>[2x]S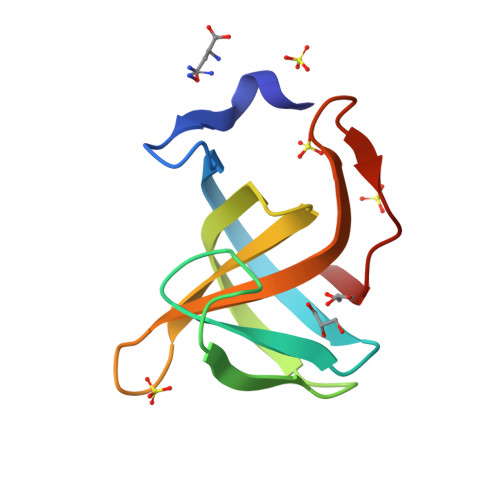NATYKVDGKGTYYKAESASFTANYDIKTRLNGPFRSNPQSGVLHPGQTIKYDTVMKQDGHVWVVYTGYSGKRIYLPVRTWDKNSNTLGPLWGIIN> ANLNGTLMQYFEWYMPNDGQHWKRLQNDSAYLAEHGITAVWIPPAYKGTSQADVGYGAYDLYDLGEFHQKGTVRTKYGTKGELQSAIKSLHSRDINVYGDVV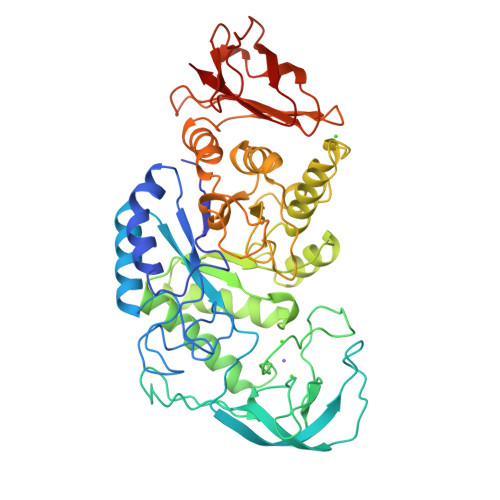INHKGGADATEDVTAVEVDPADRNRVISGEHLIKAWTHFHFPGRGSTYSDFKWHWYHFDGTDWDESRKLNRIYKFQGKAWDWEVSNEFGNYDYLMYADIDYDHPDVAAEIKRWGTWYANELQLDGFRLDAVKHIKFSFLRDWVNHVREKTGKEMFTVAEYWSYDLGALENYLNKTNFNHSVFDVPLHYQFHAASTQGGGYDMRKLLNGTVVSKHPLKSVTFVDNHDTQPGQSLESTVQTWFKPLAYAFILTRESGYPQVFYGDMYGTKGDSQREIPALKHKIEPILKARKQYAYGAQHDYFDHHDIVGWTREGDSSVANSGLAALITDGPGGAKRMYVGRQNAGETWHDITGNRSEPVVINSAGWGEFHVNGGSVSIYVQR The recently identified plasmid-encoded MCR-1 enzyme is the first transmissible colistin resistance determinant and is a cause for concern for the spread of this resistance trait. MCR-1 is a phosphoethanolamine transferase that catalyzes the addition of phosphoethanolamine to lipid A to decrease colistin affinity. The location of the catalytic domain of full-length MCR-1 is presumably on the periplasmic face of the cytoplasmic membrane, based on the predicted five membrane spanning helices in the N-terminal transmembrane domain of the protein and previous results with PEA transferases. The catalytic domain of MCR-1 assumes the α/β/α fold characteristic of the alkaline phosphatase superfamily.

Here, we report the X-ray crystal structure of the soluble, periplasmic catalytic domain of the MCR-1 enzyme determined at 1.32 Å resolution. The cMCR-1 protein crystallized in the P43212 space group with one molecule in the asymmetric unit. cMCR-1 is a globular protein with an overall hemispherical shape and a centrally located β-sheet composed of seven β-strands sandwiched between α-helical structures. The biological function of the enzyme and the tetrahedral shape of the density suggested the presence of a phosphate group covalently attached to the side-chain oxygen resulting from phosphorylation of Thr285. Surrounding the phosphothreonine are three zinc ions, which were identified by the anomalous signal and further confirmed by difference maps. Zn1 is buried in the active site of MCR-1 and is tetrahedrally coordinated by a phosphate oxygen of phosphothreonine-285 as well as the conserved residues Asp465, Glu246, and His466. Zn2 is bound by a phosphate oxygen of phosphothreonine-285, Nε2 atom of His395, and three waters in a trigonal bipyramidal configuration. Finally MCR-1 contains a third zinc that contacts phosphothreonine-285 but is not coordinated by other MCR-1 residues and a fourth zinc that is bridged by a neighboring MCR-1 molecule in the crystal lattice. The peripheral location of these zincs suggests they may not play a role in catalysis and may be a function of the high zinc concentration in the crystallization conditions for MCR-1. The catalytic domain of MCR-1 contains six cysteine residues and the cysteines form three disulfide bonds between residues Cys281/Cys291, Cys356/Cys364, and Cys414/Cys422.

> HHHHHHENLYFQHMSAPKDTIYHAKDAVQATKPDMRKPRLVVFVVGETARADHVSFNGYERDTFPQLAKIDGVTNFSNVTSCGTSTAYSVPCMFSYLGADEYDVDTAKYQENVLDTLDRLGVSILWRDNNSDSKGVMDKLPKAQFADYKSATNNAICNTNPYNECRDVGMLVGLDDFVAANNGKDMLIMLHQMGNHGPAYFKRYDEKFAKFTPVCEGNELAKCEHQSLINAYDNALLATDDFIAQSIQWLQTHSNAYDVSMLYVSDHGESLGENGVYLHGMPNAFAPKEQRSVPAFFWTDKQTGITPMATDTVLTHDAITPTLLKLFDVTADKVKDRTAFIR>[4x]GDTKEQRILRYVQQ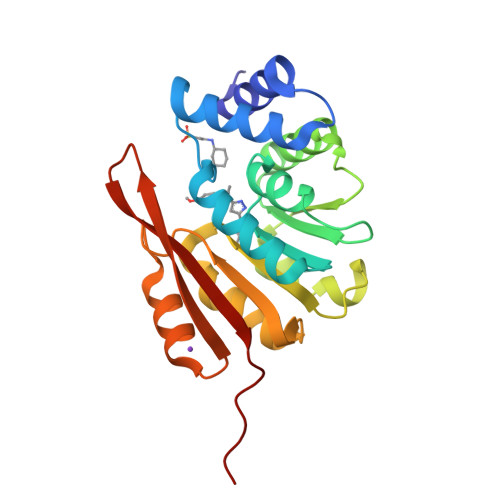NAKPGDPQSVLEAIDTYCTQKEWAMNVGDAKGQIMDAVIREYSPSLVLELGAYCGYSAVRMARLLQPGARLLTMEINPDCAAITQQMLNFAGLQDKVTILNGASQDLIPQLKKKYDVDTLDMVFLDHWKDRYLPDTLLLEKCGLLRKGTVLLADNVIVPGTPDFLAYVRGSSSFECTHYSSYLEYMKVVDGLEKAIYQGPSSPDK> MEGVAMEDI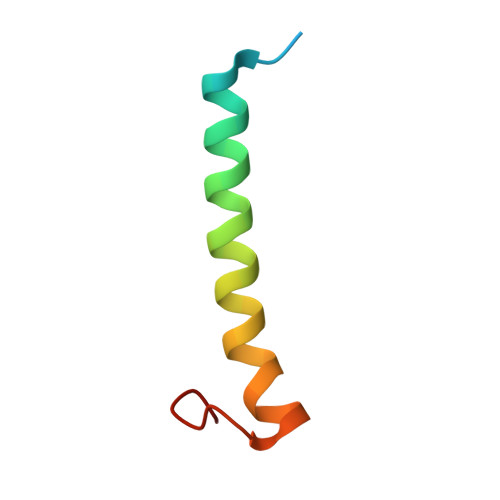SKVAWAWFGVLLAICLIGAFGNYVPKLFVKMLMFLN> LEEKKVCQGTSNKLTQLGTFEDHFLS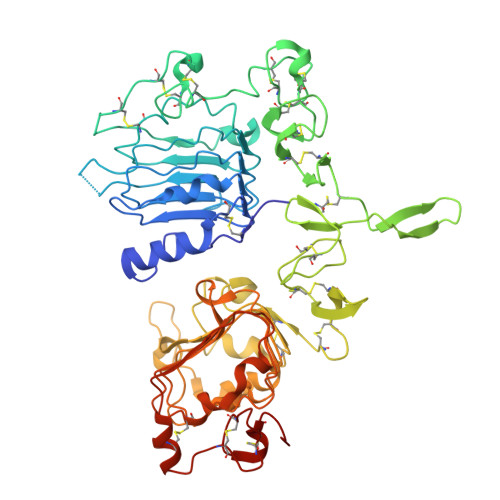LQRMFNNCEVVLGNLEITYVQRNYDLSFLKTIQEVAGYVLIALNTVERIPLENLQIIRGNMYYENSYALAVLSNYDANKTGLKELPMRNLQEILHGAVRFSNNPALCNVESIQWRDIVSSDFLSNMSMDFQNHLGSCQKCDPSCPNGSCWGAGEENCQKLTKIICAQQCSGRCRGKSPSDCCHNQCAAGCTGPRESDCLVCRKFRDEATCKDTCPPLMLYNPTTYQMDVNPEGKYSFGATCVKKCPRNYVVTDHGSCVRACGADSYEMEEDGVRKCKKCEGPCRKVCNGIGIGEFKDSLSINATNIKHFKNCTSISGDLHILPVAFRGDSFTHTPPLDPQELDILKTVKEITGFLLIQAWPENRTDLHAFENLEIIRGRTKQHGQFSLAVVSLNITSLGLRSLKEISDGDVIISGNKNLCYANTINWKKLFGTSGQKTKIISNRGENSCKATGQVCHALCSPEGCWGPEPRDCVSHHHHHH>MGSSHHHHHHSSGRENLYFQGHMAGRRRWSTEQILDAAAELLLAGDAETFSVRKLAASLGTDSSSLYRHFRNKTELLRAVADRILLSAMDGYRPEGDWKQRLTAVALRLRESFGQQPQLAAVWGRHGSGGTGSRLMMEEVLQALRASGLPDDEIPARYHRLVILISSLITAEGGFGAVGAQEH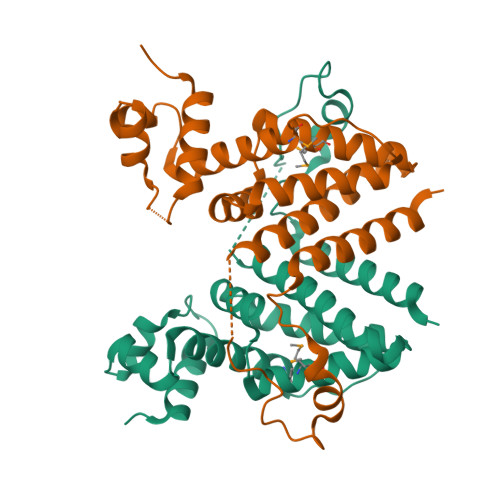EQGMEQFRVAVLGADPERFPALSHFAREIRPLGADRGAAFEEILAAHLAHLEAAAPGS[2x]> T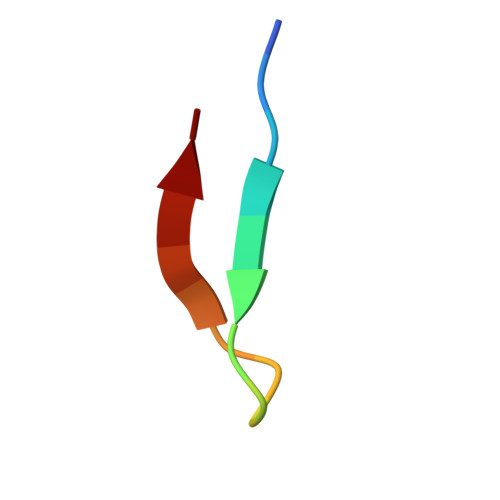SSKIYDNKNQLIADL>MGEDDKLKRMFSWSSNALSEGSAMGERVEPVVPGPDLVGVNVERPPAPLVHQQSTVWSKRQHAVCVRHAFKQYGSKKNPNHVLSDLNMTVAKGTIYGLLGASGCGKTTLLSCIVGRRRLNTGEIWVLGGKPGTKGSGVPGKRVGYMPQEIALYGEFSIKETMMYFGWIFGMESSEINERLQFLLNFLDLPSQNRLVKNLSGGQQRRVSFAVALMHDPELLILDEPTVGVDPLLRQSIWNHLVQITKDGNKTVIITTHYIEEARQAHTIGLMRSGKLLAEESPHVLLSMYGCQSLEEVFLKLSRKQGQANQNDINISNNISLATLNWGKKDSISVTEESGVVGLNFHQSKEILIADSTNGHIDLNGLGKPSSSKSSMADACDDCSCSDMTSWGKIKALLQKNFLRMWRNVGVMLFIFALPVMQVILFCLAIGRDPTGLKLAIVNHEKNYTNQSYQECSFDYGCKFSYLSCRYLNNLRNSTILKEYYPDPESAVDAVKQGHAWGALYFTENFTDALVARMALGKDADPETLDQSEVRVWLDMSNQQIGIILQRDLQLSYQDFAKDLLGACEQNPDLAEIPISFKEPIYGSNKPSFTDFVAPGVILTIVFFLAVALTSSALIIERMEGLLDRSWVAGVTPGEILFSHVVTQFVVMCGQTALVLIFMILVFGVQCKGDIGWVIVLTILQGLCGMCFGFVISAICELERNAIQLALGSFYPTLLLSGVIWPIEGMPTVLRYVSTFLPLTLATTSLRAMLTRGWSIAEPAVYYGFLATIIWIVAFLTISMLVLRFKR[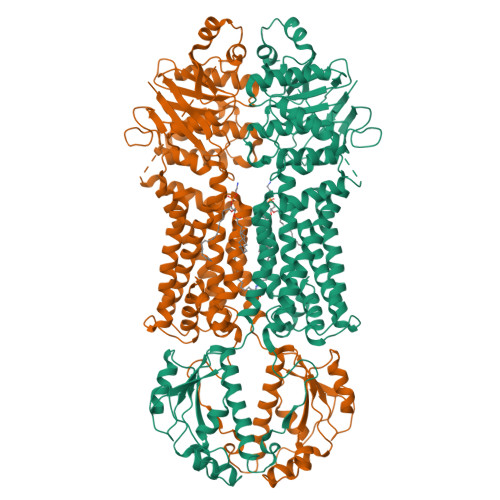2x]A plant called Arabidopsis thaliana has a light-sensitive protein called ZEITLUPE (or ZTL for short) that helps it keep its circadian clock in sync with the cycle of night and day. In Arabidopsis thaliana, three LOV domain containing proteins ZTL, FLAVIN-BINDING, KELCH REPEAT, F-BOX 1 (FKF1), and LOV KELCH PROTEIN 2 (LKP2) act in circadian timing and seasonal flowering. Recent research indicates that their divergent roles in the circadian clock and photoperiodic flowering may enable interrogation of how chemistry regulates PAS/LOV protein function to select for signaling pathways. These proteins retain analogous elements, where an N-terminal LOV domain regulates activity of a C-terminal E3 ubiquitin ligase to target clock proteins for degradation in a time dependent manner. LOV domains are typified by blue-light induced formation of a C4a adduct between a conserved Cys residue and a bound flavin (FAD, FMN or riboflavin) cofactor.

Towards these aims we solved 2.5 Å, 2.6 Å, and 2.1 Å crystal structures of dark-state WT ZTL, G80R and V48I:G80R (residues 29–165) respectively. In contrast, examination of V48I containing structures reveals distinct differences that identify allosteric signal transduction mechanisms to the N/Ccap. These mechanisms identify V48I as a residue that disrupts allosteric regulation of ZTL function. V48I positions the additional methyl group into a pocket adjacent to N5, C82 and Q154. The Q154 conformation is not heterogeneous in V48I:G80R, rather, the Ile side chain sterically directs Q154 to an exposed conformation near O4 that has not been observed in other LOV proteins. Density shows clear selection of the I48 methyl group towards Q154. Lack of density for an adduct is consistent with minimal population of the light-state species. Thus, the presence of G46 selects for a heterogeneous conformation of Q154 and V48I biases the heterogeneous Q154 towards the exposed conformation in the dark. Introduction of V48I, directs Q154 to a single exposed conformation in the dark. Biasing the Q154 to the exposed conformation results in disrupted interactions with GI and high TOC1/PRR5 degradation, in vivo, consistent with selecting for a distinct dark-state conformation.

>GGPIPYPVGNLLHTAPCGFIVTDAVEPDQPIIYVNTVFEMVTGYRAEEVLGRNCRFLQCRGPFAKRRHPLVDSMVVSEIRKCIDEGIEFQGELLNFRKDGSPLMNRLRLTPIYGDDDTITHIIGIQFFIETDIDLGP[4x]>MGSHHHHHHGRSMSELIKENMHMKLYMEGTVNNHHFKCTSEGEGKPYEGTQTMRIKVVEGGPLPFAFDILATSFMYGSRTFINHTQGIPDFWKQSFPEGFTWERVTTYEDGGVLTATQDTSLQDGCLIYNVKLRGVNFPSNGPVMQKKTLGWEAATEMLYPADGGLEGRGDMALKLVGGGHLICNLKTTYRSKNPAKNLKMPGVYFVDHRLERIKEADKETYVEQHEVAVARYCDLPSKLGHKLN[4x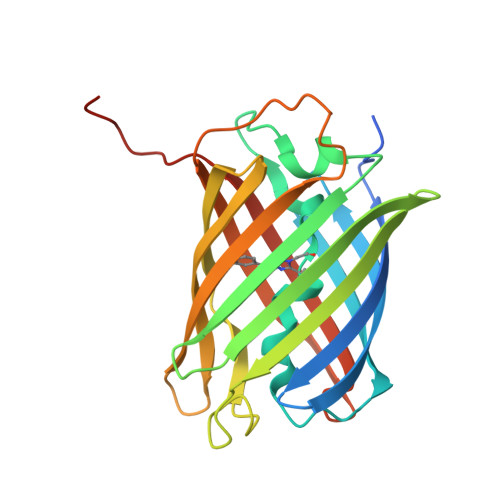]>[4x]MDNLSFRPKLYLAAPLFNEAEKESNRNIRDSLIDCCDVFLPQEDGLLLDELVSLGTPLKVAEKSIYEADI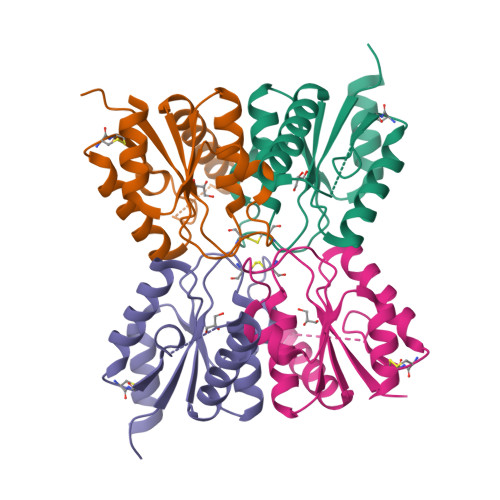SAMKNADILLAVLDGACIDDGVAFELGYAKAINKVCLGFQTDVRRQAPTGNNPMIECSCEEIFSDLGSLKKWLQQKYNKLS>MVRGIRGAITVEEDTPEAIHQATRELLLKMLEANGIQSYEELAAVIFTVTEDLTSAFPAEAARQIGMHRVPLLSAREVPVPGSLPRVIRVLALWNTDT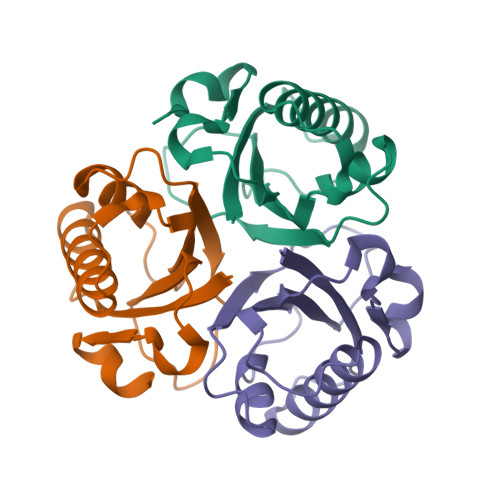PQDRVRHVYLREAVRLRPDLESAQ[3x]> MVAPEHRVLHLRDRLDLAAELKLLCERGPLVRIPLEDGSAVHWFALGYDVVREVLGSEKFDKRVIGTHFNHQEMALPGNLLQLDPPEHTRLRRMVAPAYSVRRMQALEPRVQAIVDDHLDTMASTGPPVEFLREVAGPMAARVACEFLGIPLDDRGELIRLTAHRGGKRRRVLNGHAYLAYMRELAARLRRDPGDGMLGMVARDHGADISDEELAGLCAVVMNSSVEQTESCLAAGTLLLLEHPEQFALLRERPELGEQAVEEIVRYLSVFEGLDPRTATEDVEIGGQVIKKGEAVFCSLLAANRADPALDGFDITRKESRHVAFGHGIHHCLGAPLAR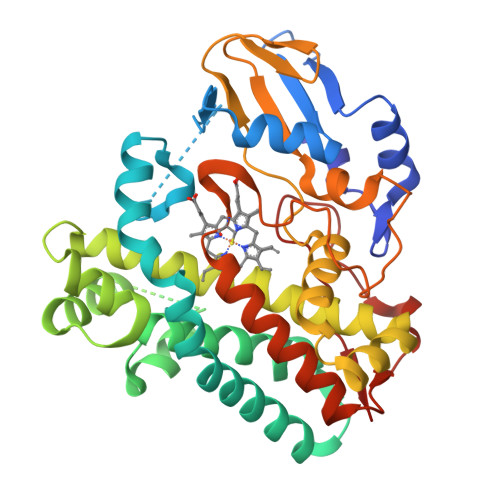MELRIAFTTLVSRFPSLRTAVPAEEIRFRPPSSNVFTLLELPLTW> QTQQEEEEEDEDHGPDDYDEEDEDEVEEEETNRLPGGRSRVLLRCYTCKSLPRDERCNLTQNCSHGQTCTTLIAHGNTESGLLTTHSTW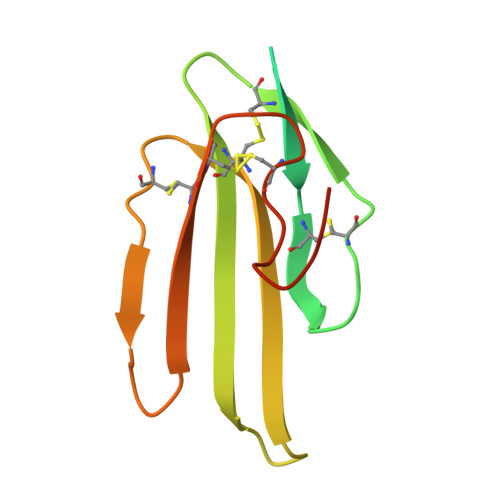CTDSCQPITKTVEGTQVTMTCCQSSLCNVPPWQSSRVQDPTG> MSAYATQGFNLDDRGRRIVVDPVTRIEGHMRCEVNVDANNVIRNAVSTGTMWRGLEVILKGRDPRDAWAFVERICGVCTGCHALASVRAVENALDIRIPKNAHLIREIMAKTLQVHDHAVHFYHLHALDWVDVMSALKADPKRTSELQQLVSPAHPLSSAGYFRDIQNRLKRFVESGQLGPFMNGYWGSKAYVLPPEANLMAVTHYLEALDLQKEWVKIHTIFGGKNPHPNYLVGGVPCAINLDGIGAASAPV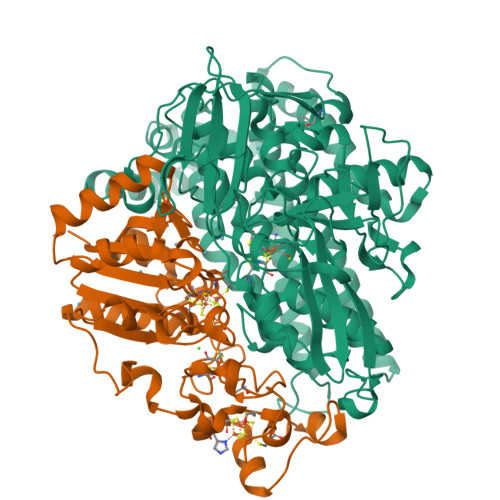NMERLSFVKARIDEIIEFNKNVYVPDVLAIGTLYKQAGWLYGGGLAATNVLDYGEYPNVAYNKSTDQLPGGAILNGNWDEVFPVDPRDSQQVQEFVSHSWYKYADESVGLHPWDGVTEPNYVLGANTKGTRTRIEQIDESAKYSWIKSPRWRGHAMEVGPLSRYILAYAHARSGNKYAERPKEQLEYSAQMINSAIPKALGLPETQYTLKQLLPSTIGRTLARALESQYCGEMMHSDWHDLVANIRAGDTATANVDKWDPATWPLQAKGVGTVAAPRGALGHWIRIKDGRIENYQCVVPTTWNGSPRDYKGQIGAFEASLMNTPMVNPEQPVEILRTLHSFDPCLACSTH;> METKPRTPVLWLHGLECTCCSESFIRSAHPLAKDVVLSMISLDYDDTLMAAAGHQAEAILEEIMTKYKGNYILAVEGNPPLNQDGMSCIIGGRPFIEQLKYVAKDAKAIISWGSCASWGCVQAAKPNPTQATPVHKVITDKPIIKVPGCPPIAEVMTGVITYMLTFDRIPELDRQGRPKMFYSQRIHDKCYRRPHFDAGQFVEEWDDESARKGFCLYKMGCKGPTTYNACSTTRWNEGTSFPIQSGHGCIGCSEDGFWDKGSFYDRLTGISQFGVEANADKIGGTASVVVGAAVTAHAAASAIKRASKKNETSGSEHRSAWSHPQFEKRSAWSHPQFEK> PREPRPNEECLQILGNAEKGAKFLSDAEIIQLVNAKHIPAYKLETLMETHERGVSIRRQLLSKKLSEPSSLQYLPYRDYNYSLVMGACCENVIGYMPIPVGVAGPLCLDEKEFQVPMATTEGCLVASTNRGCRAIGLGGGASSRVLADGMTRGPVVRLPRACDSAEVKAWLETSEGFAVIKEAFDSTSRFARLQKLHTSIAGRNLYIRFQSRSGDAMGMNMISKGTEKALSKLHEYFPEMQILAVSGNYCTDKKPAAINWIEGRGKSVVCEAVIPAKVVREVLKTTTEAMIEVNINKNLVGSAMAGSIGGYNAHAANIVTAIYIACGQDAAQNVGSSNCITLMEASGPTNEDLYISCTMPSIEIGTVGGGTNLLPQQACLQMLGVQGACKDNPGENARQLARIVCGTVMAGELSLMAALAAGH

The rate-limiting enzyme 3-hydroxy-3-methylglutaryl-coenzyme A (HMG-CoA) reductase (HMGR) catalyses the reduction of HMG-CoA to mevalonate and tightly regulates the level of cholesterol in humans. Therefore, the human enzyme (hHMGR) has been identified as a potent natural target for hypercholesterolemia diseases resulting from higher levels of cholesterol. For the atorvastatin-bound form and from the apo structure in this report, the catalytic part of hHMGR forms a homotetramer comprising two homodimers arranged in D2 symmetry. The two neighbouring monomers of the dimer contribute residues to form an active site and hence there are four active sites per tetrameric complex.

To our knowledge, the apo structure of the human enzyme has previously not been reported; we describe the structure at 2.1 Å resolution and compare it with the inhibitor atorvastatin-bound form. Here, we used SPA cryo-EM to solve the structures of the apo and atorvastatin-bound forms of the catalytic domain of the important pharmaceutical target hHMGR at atomic resolution by exploiting graphene oxide as an additional support on the holey carbon grids. Secondly, to reduce the high background contrast from the glycerol in the buffer component and additionally from DMSO for the atorvastatin-bound sample, the grid was washed with buffer lacking glycerol prior to vitrification. Overall, our approach increased the contrast in the images sufficiently to obtain near-atomic resolution reconstructions of apo hHMGR and the atorvastatin-bound complex at 2.1 and 2.3 Å resolution, respectively, from particles adopting a slightly preferred orientation. In all crystal structures reported to date, a region of N-terminal N-domain residues 439–487 was found to be highly flexible and therefore was only partially modelled. Notably, in both the apo and atorvastatin-bound cryo-EM structures the entire region can be modelled as the density is clearer.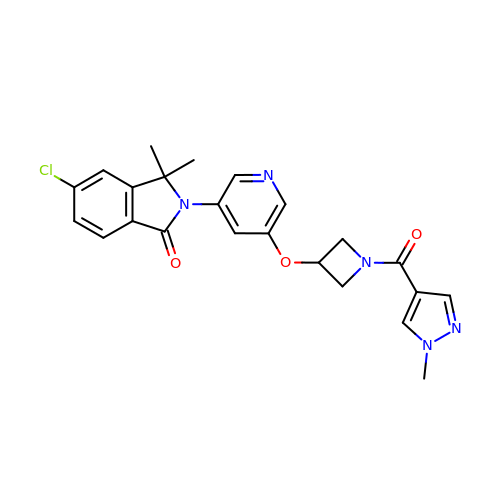5-chloranyl-3,3-dimethyl-2-[5-[1-(1-methylpyrazol-4-yl)carbonylazetidin-3-yl]oxypyridin-3-yl]isoindol-1-one | C23 H22 Cl N5 O3 | UBYILWVEJSMRTQ-UHFFFAOYSA-N>[3x]MGSDKIHHHHHHMRLYTRTGDKGKTSVIGGRLAKDDTRVVAYGTTDELNSF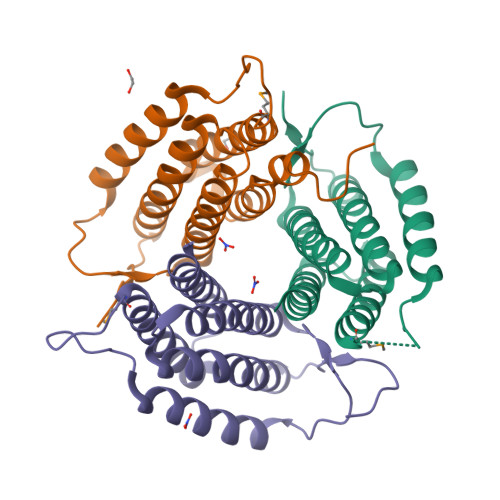VGSAITQLDENTFADIRGELFKIQHELFDCGGDLAMLKVKEDRPYKAKQEIVDFLEQRIDAYIKEAPELERFILPGGSEAAASLHVCRTIARRAERYVVRLQQEGEINPIVLKYLNRLSDYFFAVARVVNSRLQVPDVEYERSAIVFREGKRKEDKK>[2x]GCD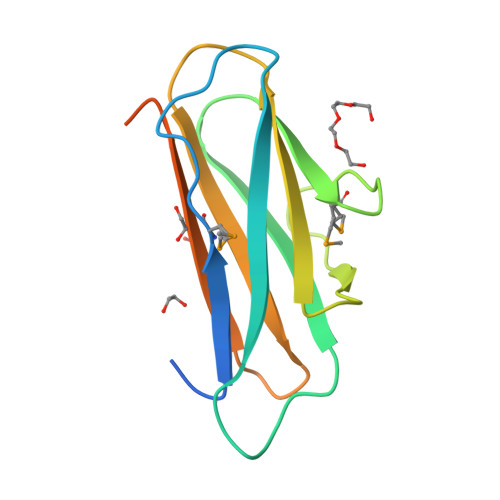DDMDIQQSYPFTVEVMPVPNKVVKGQTVEIRCELKKEGDFSGTLYTIRYFQFEGEGSLKMDNGITFLPNDRYLLENEKFRLYYTAAGDEAHNFIVVVEDNFSNSYELEFDFNNRNVKDDDLTIVPIGNFSPLLK(1,5-dimethylpyrazol-4-yl)methyl (2~{S})-1-[(2~{S})-2-cyclohexyl-2-(3,4,5-trimethoxyphenyl)ethanoyl]piperidine-2-carboxylate | C29 H41 N3 O6 | 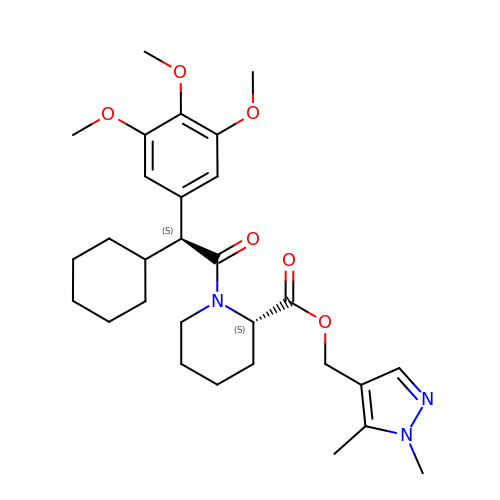PSPZXGLIXLRMAD-OZXSUGGESA-N>MGGSHHHHHHGDDDDKMTKDFRQNVFQGRSVLAEKDFSAAELEYLIDFGLHLKALKKAGIPHHYLEGKNIALLFEKSST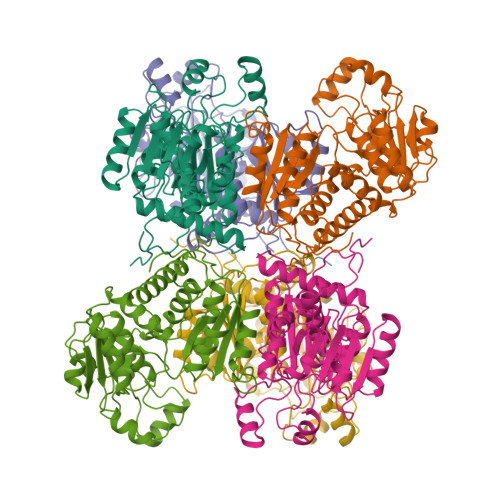RTRSAFTTASIDLGAHPEYLGQNDIQLGKKESTSDTAKVLGSMFDGIEFRGFKQSDAEILARDSGVPVWNGLTDEWHPTQMLADFMTVKENFGKLQGLTLTFMGDGRNNVANSLLVTGAILGVNIHIVAPKALFPTEETQNIAKGFAEKSGAKLVITDDLDEGLKGSNVVYTDVWVSMGESNWEERVKELTPYQVNMEAMKKTGTPDDQLIFMHCLPAFHNTDTQYGKEIKEKYGITEMEVTDEVFTSKYARQFEEAENRMHSIKAMMAATLGNLFIPRV[3x]benzenesulfonic 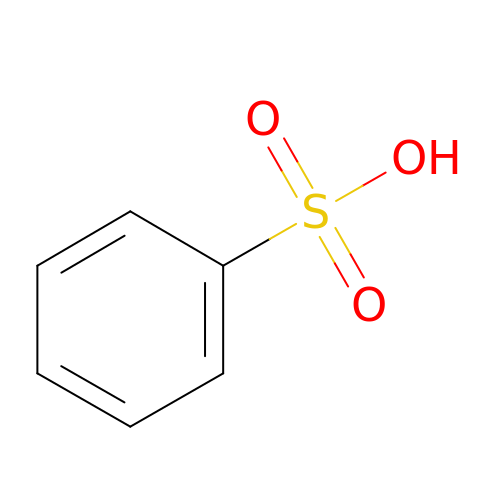acid | C6 H6 O3 S | SRSXLGNVWSONIS-UHFFFAOYSA-N ethyl 2-(2-{2-[(1S)-1-amino-4-carbamimidamidobutyl]-1,3-thiazol-4-yl}-5-methyl-1,3-oxazol-4-yl)-1,3-thiazole-4-carboxylate 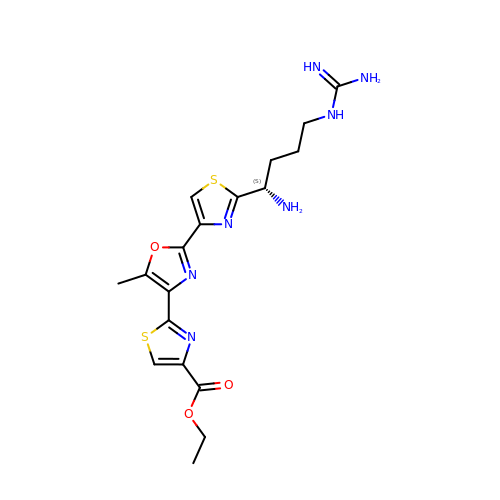| C18 H23 N7 O3 S2 | LDXVRBOROSJVJC-JTQLQIEISA-N> MVKIYLIEHVIGAVAYDENGNIVDYITNPRDLGKITEELLNNEKGIPFSATVELLKKVNPQEVVVENEAEVPKLQALGYRVSYEPYSKVSRIFRESLPKVAIDIKFASNEEDYYNFLHELSLEYTRRKLRSAAQKRDLLAIQAVRAMDDIDKTINLFSERLREWYSIHFPELDKLIEDHEEYATIVSRFGDRGFLTIDSLKELGFNEQRINRILDAAKKSIGADISEDDLSAMRMIANTILDLYNIRRNLNNYLEGVMKEVAPNVTALVGPALGARLLSIAGSLDELAKMPASTIQVLGAEKALFRALRSGGRPPKHGIIFQYPAIHTSPRWQRGKIARALAAKLAIAARVDAFSGRFIGDQLNEQLKKRIDEIKEK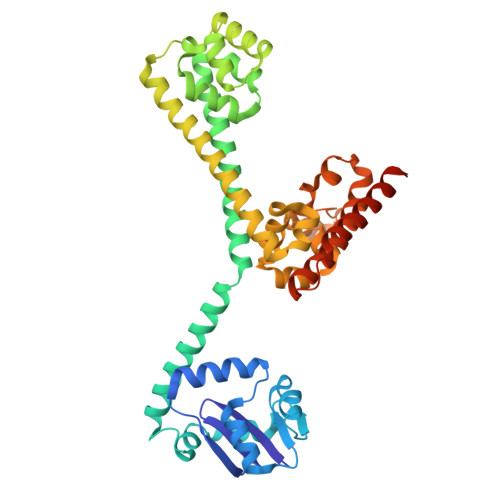FAQHHHHHHHH>[2x]GSHMSLSNKLTLDKLDVKGKRVVMRVDFNVPMKNNQITNNQRIKAAVPSIKFCLDNGAKSVVLMSHLGRPDGVPMPDKYSL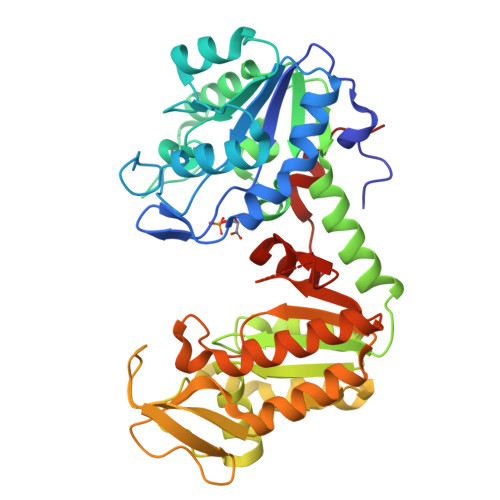EPVAVELKSLLGKDVLFLKDCVGPEVEKACANPAAGSVILLENLRFHVEEEGKGKDASGNKVKAEPAKIEAFRASLSKLGDVYVNDAFGTAHRAHSSMVGVNLPQKAGGFLMKKELNYFAKALESPERPFLAILGGAKVADKIQLINNMLDKVNEMIIGGGMAFTFLKVLNNMEIGTSLFDEEGAKIVKDLMSKAEKNGVKITLPVDFVTADKFDENAKTGQATVASGIPAGWMGLDCGPESSKKYAEAVTRAKQIVWNGPVGVFEWEAFARGTKALMDEVVKATSRGCITIIGGGDTATCCAKWNTEDKVSHVSTGGGASLELLEGKVLPGVDALSNI Notwithstanding this diversity colicins invariably have a similar domain arrangement, where a central receptor-binding (R) domain is flanked by an N-terminal translocation (T) domain and a C-terminal cytotoxic (C) domain. E-type colicins parasitize the vitamin B12 receptor, BtuB, as their primary receptor in the outer membrane and the Tol-Pal complex in the periplasm. The catalytic centre of most colicin and pyocin DNases is the HNH/ββα-Me motif, a 34-amino acid motif containing invariant histidine residues, which chelates a single divalent metal ion that catalyzes phosphodiester bond hydrolysis. DNase-specific Im proteins are small acidic inhibitors that bind to an exosite and inhibit colicin or pyocin activity indirectly by blocking substrate-binding.

We therefore switched to using a disulphided form of ColE9 in which Tyr324 and Leu447 in the R-domain were mutated to cysteine, which has been reported previously. We obtained X-ray diffracting crystals of this disulphide locked form of the ColE9–Im9 complex in the P21 space group, and the structure was refined to a resolution of 3.2 Å. The asymmetric unit contains four ColE9–Im9 complexes, two pairs of molecules related by non-crystallographic two-fold symmetry. The final model of the ColE9–Im9 complex contains 488 residues of ColE9 (85–580) and 83 residues of Im9 (3–85). No electron density was visible for the first 84 N-terminal residues of ColE9 that comprise the intrinsically unstructured translocation domain (IUTD) of the colicin, consistent with nuclear magnetic resonance spectroscopy data showing that this domain is disordered. As with other colicins (ColE3 and the pore-forming toxin ColIa), ColE9 adopts an extended structure with overall dimensions of 130 × 75 × 35 Å. In the present structure, however, no additional electron density was observed in the HNH motif, suggesting that no metal ion is bound within the catalytic centre. Our structure for the ColE9–Im9 complex, only the second intact colicin nuclease structure after the ColE3–Im3 complex, shows how the conserved scaffold of T- and R-domains presents the E9 DNase–Im9 complex in a different orientation to that of the E3 rRNase–Im3 complex where the Im protein is sandwiched between the T- and C-domains. The result of these differences is that the DNase domain of ColE9 is rotated ∼90° away from the T-domain relative to ColE3, which is emphasized by the 12 Å movement of equivalent Cα atoms in the structural superposition of the two colicins. The lack of an interaction with the T-domain explains why the affinity of Im9 for ColE9 and the isolated E9 DNase are identical.

>MSGGDGRGHNTGAHSTSGNINGGPTGIGVSGGASDGSGWSSENNPWGGGSGSGIHWGGGSGRGNGGGNGNSGGGSGTGGNLSAVAAPVAFGFPALSTPGAGGLAVSISASELSAAIAGIIAKLKKVNLKFTPFGVVLSSLIPSEIAKDDPNMMSKIVTSLPADDITESPVSSLPLDKATVNVNVRVVDDVKDERQNISVVSGVPMSVPVVDAKPTERPGVFTASIPGAPVLNISVNDSTPAVQTLSPGVTNNTDKDVRPAGFTQGGNTRDAVIRFPKDSGHNAVYVSVSDVLSPDQVKQRQDEENRRQQEWDATHPVEAAERNCERARAELNQANEDVARNQERQAKAVQVYNSRKSELDAANKTLADAIAEIKQFNRFAHDPMAGGHRMWQMAGLKAQRAQTDVNNKQAAFDAAAKEKSDADAALSAAQERRKQKENKEKDAKDKCAMESKRNKPGKATGKGKPVGDKWLDDAGKDSGAPIPDRIADKLRDKEFKSFDDFRKAVWEEVSKDPELSKNLNPSNKSSVSKGYSPFTPKNQQVGGRKVYELHHDKPISQGGEVYDMDNIRVTTPKRHIDIHRGK[4x];>[4x]MELKHSISDYTEAEFLQLVTTICNADTSSEEELVKLVTHFEEMTEHPSGSDLIYYPKEGDDDSPSGIVNTVKQWRAANGKSGFKQGLEHHHHHH>[2x]MKHSHEEIRKIIPEMRRVQQIHFIGIGGAGMSGIAEILLNEGYQISGSDIADGVVTQRLAQAGAKIYIGHAEEH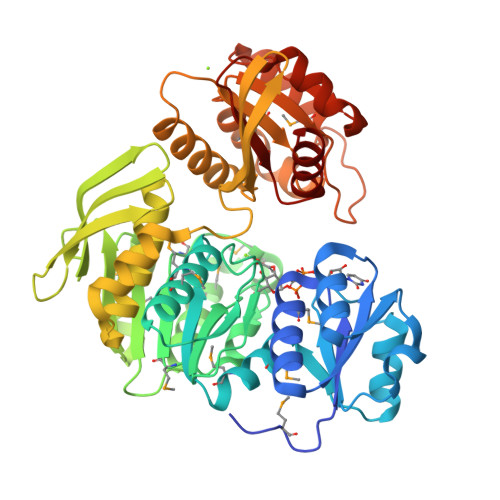IEGASVVVVSSAIKDDNPELVTSKQKRIPVIQRAQMLAEIMRFRHGIAVAGTHGKTTTTAMISMIYTQAKLDPTFVNGGLVKSAGKNAHLGASRYLIAEADESDASFLHLQPMVSVVTNMEPDHMDTYEGDFEKMKATYVKFLHNLPFYGLAVMCADDPVLMELVPKVGRQVITYGFSEQADYRIEDYEQTGFQGHYTVICPNNERINVLLNVPGKHNALNATAALAVAKEEGIANEAILEALADFQGAGRRFDQLGEFIRPNGKVRLVDDYGHHPTEVGVTIKAAREGWGDKRIVMIFQPHRYSRTRDLFDDFVQVLSQVDALIMLDVYAAGEAPIVGADSKSLCRSIRNLGKVDPILVSDTSQLGDVLDQIIQDGDLILAQGAGSVSKISRGLAESWKN S-ADENOSYL-1,8-DIAMINO-3-THIOOCTANE 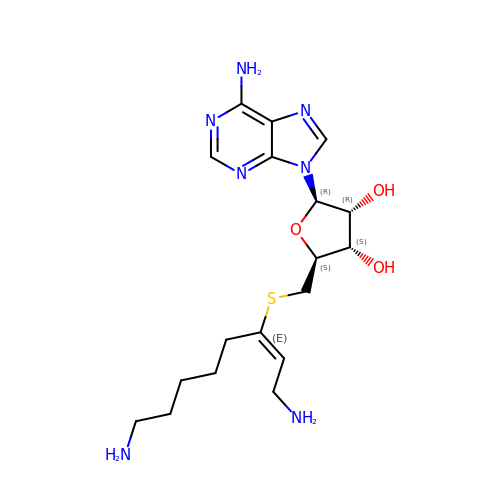| C18 H29 N7 O3 S | SUUGLGYBZXSJAA-SCFUHWHPSA-N>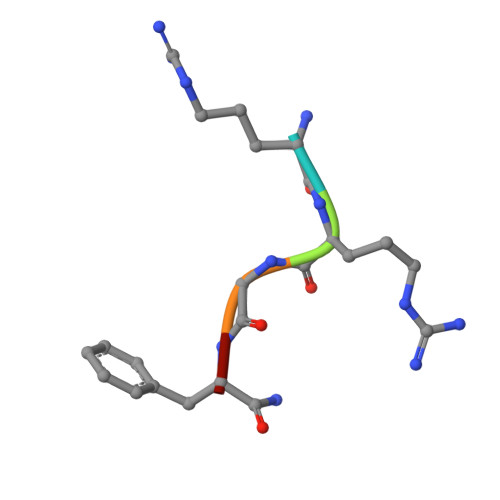 RRGFX> GSPCPGA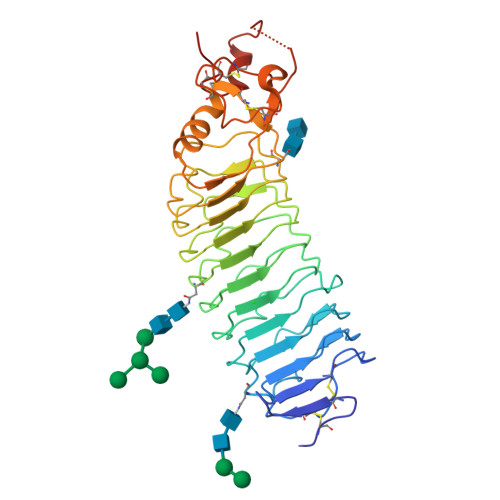CVCYNEPKVTTSCPQQGLQAVPTGIPASSQRIFLHGNRISHVPAASFQSCRNLTILWLHSNALARIDAAAFTGLTLLEQLDLSDNAQLHVVDPTTFHGLGHLHTLHLDRCGLRELGPGLFRGLAALQYLYLQDNNLQALPDNTFRDLGNLTHLFLHGNRIPSVPEHAFRGLHSLDRLLLHQNHVARVHPHAFRDLGRLMTLYLFANNLSMLPAEVLMPLRSLQYLRLNDNPWVCDCRARPLWAWLQKFRGSSSEVPCNLPQRLADRDLKRLAASDLEGCAVASGPFRPIQTSQLTDEELLSLPKCCQAAAHHHHHH> MAHHHHHHMLPSIAKHAASHQIHPLKKHGQNFIFDGSLCDKIVRASGLEENSNVLEIGPGTGGLTRSILHKNPKLLTVIETDERCIPLLNEIKQYHPNLNIIKQDALKLKLSDLNTNKITIISNLPYH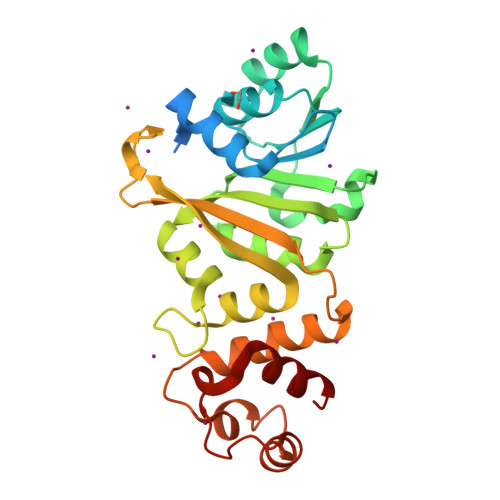IGTELVIRWLKESSLVASMTLMLQKEVVERICAKPSTKAYGRLSVICSLIATVEKCFDVAPTAFYPPPKVYSAIVKLTPLENIPNSDLISKVELITKMAFAGRRKMIKSSLKNLAPNISELLAKLNISDNCRAENLTPNDYLSLASLI> GAMGSGASFVQIKFDDLQFFENCGGGSFGSVYRAKWISQDKEVAVKKLLKIEKEAEILSVLSHRNIIQFYGVILEPPNYGIVTEYASLGSLYDYINSNRSEEMDMDHIMTWATDVAKGMHYLHMEAPVKVIHRDLKSRNVVIAADGVLKICDFGASRFHNHTTHMSLVGTFPWMAPEVIQSLPVSETCDTYSYG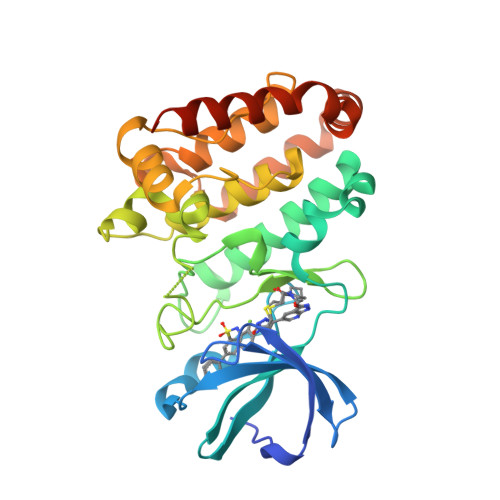VVLWEMLTREVPFKGLEGLQVAWLVVEKNERLTIPSSCPRSFAELLHQCWEADAKKRPSFKQIISILESMSNDTSLPDKCNSFLHNKAEWRCEIEATLERLKKLERDLSFKEQELK> MTKPLDGINVLDFTHVQAGPACTQMMGFLGANVIKIERRGSGDMTRGWLQDKPNVDSLYFTMFNCNKRSIELDMKTPEGKELLEQMIKKADVMVENFGPGALDRMGFTWEYIQELNPRVILASVKGYAEGHANEHLKVYENVAQCSGGAAATTGFWDGPPTVSGAALGDSNSGMHLMIGILAALEIRHKTGRGQKVAVAMQDAVLNLVRIKLRDQQRLERTGILAEYPQAQPNFAFDRDGNPLSFDNITSVPRGGNAGGGGQPGWMLKCKGWETDADSYVYFTIAANMWPQICDMIDKPEWKDDPAYNTFEGRVDKLMDIFSFIETKFADKDKFEVTEWAAQYGIPCGPVMSMKELAHDPSLQKVGTVVEVVDEIRGNHLTVGAPFKFSGFQPEITRAPLLGEHTDEVLKELGLDDAKIKELHAKQVV;> MTKPLDGINVLDFTHVQAGPACTQMMGFLGANVIKIERRGSGDMTRGWLQDKPNVDSLYFTMFNCNKRSIELDMKTPEGKELLEQMIKKADVMVENFGPGALDRMGFTWEYIQELNPRVILASVKGYAEGHANEHLKVYENVAQCSGGAAATTGFWDGPPTVSGAALGXSNSGMHLMIGILAALEIRHKTGRGQKVAVAMQDAVLNLVRIKLRDQQRLERTGILAEYPQAQPNFA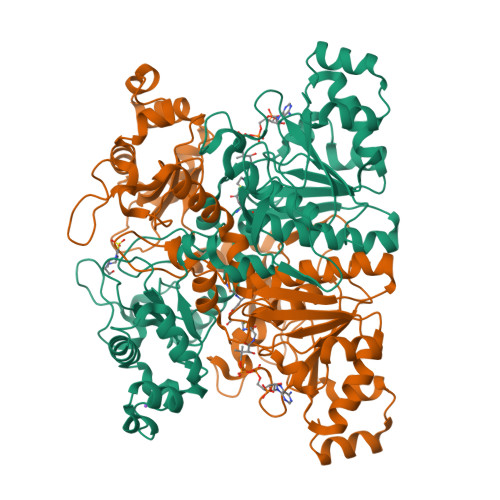FDRDGNPLSFDNITSVPRGGNAGGGGQPGWMLKCKGWETDADSYVYFTIAANMWPQICDMIDKPEWKDDPAYNTFEGRVDKLMDIFSFIETKFADKDKFEVTEWAAQYGIPCGPVMSMKELAHDPSLQKVGTVVEVVDEIRGNHLTVGAPFKFSGFQPEITRAPLLGEHTDEVLKELGLDDAKIKELHAKQVV>[11x]MASWSHPQFEKIEGRMSVTVPNDDWTLSSLSETFDDGTQTLQGELTLALDKLAKNPSNPQLLAEYQSKLSEYTLYRNAQSNTVKVIKDVDAAIIQNFR;>MLSDMSLIATLSFFTLLPFLVAAGTCYIKFSIVFVMVRNALGLQQVPSNMTLNGIALIMALFVMKPIIEAGYENYLNGPQKFDTISDIVRFSDSGLMEYKQYLKKHTDLELARFFQRSEEENADLKSAENNDYSLFSLLPAYALSEIKDAFKIGFYLYLPFVVVDLVISSILLALGMMMMSPITISVPIKLVLFVALDGWGILSKALIEQYINIPA[5x];> MDISSWFESIHVFLILLNGVFFRLAPLFFFLPFLNNGIISPSIRIPVIFLVASGLITSGKVDIGSSVFEHVYFLMFKEIIVGLLLSFCLSLPFWIFHAVGSIIDNQRGATLSSSIDPANGVDTSELAKFFNLFSAVVFLYSGGMVFILESIQLSYNICPLFSQCSFRISNILTFLTLLASQAVILASPVMIVLLLSEVLLGVLSRFAPQMNAFSVSLTIKSLLAIFIIFICSSTIYFSKVQFFLGEHKFFTNLFVR;>[5x]MSDIVYMGNKALYLILIFSLWPVGIATVIGLSIGLLQTVTQLQEQTLPFGIKLIGVSISLLLLSGWYGEVLLSFCHEIMFLIKSGV

Shigella causing dysentery utilizes the type 3-secretion system (T3SS) to inject virulence factors into the gut cells. The T3SS needle complex is a syringe-shaped nanomachine consisting of two membrane-embedded ring systems that sheath a central export apparatus and a hollow needle-like structure through which the virulence factors are transported. The T3SS structural core is a membrane-embedded transporter called needle complex, which is an evolutionary conserved syringe-like multiprotein assembly with a molecular weight of about 3.5 MDa. This complex is made of a basal body and a hollow needle that extends from the bacterial surface. The basal body is assembled by the stepwise incorporation of multiple copies of inner- (MxiG and MxiJ in Shigella) and outer- (MxiD in Shigella, which belongs to the family of the secretins) membrane proteins to form their respective rings in the corresponding membranes and periplasm.

The C1 map of the needle complex shows distinct tubular densities at the resolution of 5–6 Å in both the export apparatus and the inner rod and needle, suggesting the presence of α-helices. We used the recently published cryo-EM structure of the isolated export apparatus core from the Salmonella flagellar system as templates for modeling the structures of the Shigella proteins SpaP, SpaQ and SpaR. Random search followed by rigid body and flexible fitting allowed us to place five subunits of SpaP and SpaQ, respectively, and one of SpaR into our C1 map. Five helically arranged SpaP-SpaQ dimers build a turn terminated on the top by one SpaR, which has been suggested to resemble the fusion between SpaP and SpaQ. Analysis of the helical parameters indicates a helix pitch of 19.8 Å and 5.8 subunits per turn, similar to the parameters reported for the Salmonella flagellar complex and for the Shigella needle filament. We found evidence in our map for a 5:5:1 stoichiometry of the export apparatus proteins SpaP:SpaQ:SpaR of the Shigella T3SS. Comparison of our structure with the isolated export apparatus showed different conformation at the inner rod interface, where the N-terminal helix of a SpaP subunit occludes the opening in the isolated export apparatus, while it is bent and moved aside in the needle complex. We built a model for the inner rod fitting in our map a few turns of the published Shigella needle structure obtained by solid state NMR and EM. The inner rod has the same right-handed helical architecture as the needle with eleven subunits per two turns. We modeled the eleven subunits forming the first two turns as alanine polypeptide with helix-turn-helix conformation In vivo cross-linking studies in Salmonella have shown that PrgJ (MxiI orthologue, the inner rod subunit) interacts with SpaP and SpaR.The heterologous expression of the POD genes from the P. ostreatus genome, and subsequent kinetic studies, reveal a peroxidase array consisting of three VPs and six MnPs. The VP1 and MnP4 crystal structures were solved as representative for the two POD families present in the P. ostreatus genome. The overall structure of VP1 and MnP4 showed a heme group dividing the protein into a distal largely helical domain (formed by four main helices and two to three small ones) with one structural calcium ion, and a proximal domain composed by another six helices and a non-ordered region stabilized by a second calcium ion. The site where this takes place is conserved and comprises three acidic residues (E36/E40/D175 in VP1 and E36/E40/D181 in MnP4) located near the heme propionate occupying the most internal position with respect to the main access channel.

The resulting inventory revealed the absence of lignin peroxidases (LiPs) and the presence of three versatile peroxidases (VPs) and six manganese peroxidases (MnPs), the crystal structures of two of them (VP1 and MnP4) were solved at 1.0 to 1.1 Å showing significant structural differences. As already described for P. eryngii VPL, the main structural feature of the P. ostreatus VP1 crystal structure is the combination of the Mn oxidation site of MnPs and the high redox potential substrate oxidation site of LiPs. In addition to the Mn2+ oxidation site, VPs also present a lignin oxidation site, whose presence was detected using VA and RB5 as substrates. This site in VP1 would consist of W164, connected to the heme group via a long-range electron transfer (LRET). The indolic side chain of W164 in VP1 is largely exposed (center) allowing the collection of electrons from the bulky lignin molecule. In a similar way, the W164S mutation in VP1 resulted in a complete loss of activity on VA and RB5 (used as two simple lignin model compounds). The last change in this region concerns S180 in VP1, which is occupied by K186 in MnP4, thus affecting both the surface shape and charge. The lower lip in VP1 presents a clear negative charge and the shape of a wide reservoir, while in MnP4 it displays a less charged surface with a narrow groove (circles in Figure 5C). However, one of the main characteristics of the VP1 structure, when compared with MnP4, is the broader main heme access channel (whose lower lip has the shape of a wide reservoir), which could be related to the reported existence of a third substrate oxidation site in VP. VP1 is the most stable POD retaining over 80% activity after 10 minutes up to 60°C, followed by MnP4, VP3, MnP1, and VP2 (although the VP2 stability sharply decreased with incubation time).

> MATCADGRTTANAACCVLFPILDDIQENLFDGAQCGEEVHESLRLTFHDAIGFSPTLGGGGADGSIITFDTIETNFPANAGIDEIVSAQKPFVAKHNISAGDFIQFAGAVGVSNCPGGVRIPFFLGRPDAVAASPDHLVPEPFDSVDTILARMGDAGFSAVEVVWLLASHSIAAADKVDPSIPGTPFDSTPGVFDSQFFIETQLKGRLFPGTPDNKGEVQSPLQGEIRLQSDHLLARDPQTACEWQSMVNNQPKIQNRFAGTMSKMALLGQDKSKLIDCSDIIPTPPALVGAAHLPAGFSLSDVEQACAETPFPALTADPGPVTSVPPVPGS> MRSRRVDVMDVMNRLILAMDLMNRDDALRVTGEVREYIDTVKIGYPLVLSEGMDIIAEFRKRFGCRIIAAFKVADIPETNEKICRATFKAGADAIIVHGFPGADSVRACLNVAEEMGREVFLLTEMSHPGAEMFIQGAADEIARMGVDLG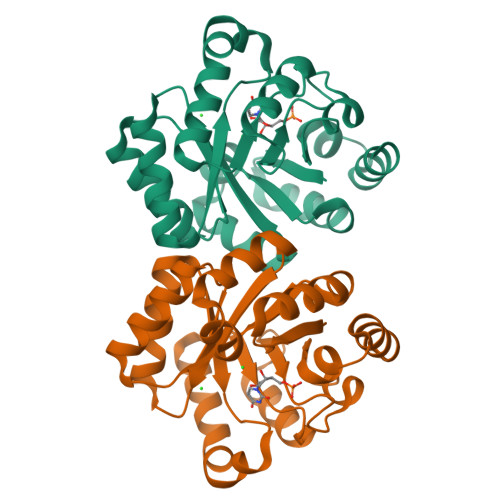VKNYVGPSTRPERLSRLREIIGQDSFLISPGVGAQGGDPGETLRFADAIIVGRSIYLADNPAAAAAGIIESIKDLLNPEDPAANKARKEAELAAATA> MLSCELYRMSTYSTFPAGVPVSERSLARA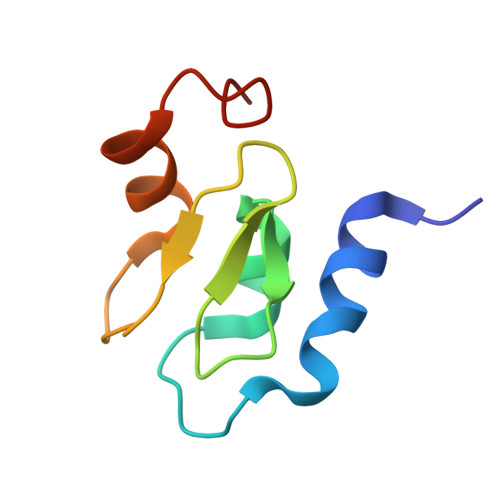GFYYTGVNDKVKCFCCGLMLDNWKRGDSPTEKHKKLYPSCRFVQSL The tripartite signalling system YfiBNR in P. aeruginosa modulates intracellular c-di-GMP levels in response to signals received in the periplasm and is a key regulator of the SCV phenotype. The effector protein YfiN (also known as TpbB or PA1120) is an integral inner membrane protein that functions as a diguanylate cyclase, consisting of a periplasmic PAS domain, a cytoplasmic HAMP domain and a catalytic GGDEF domain. The third component of the YfiBNR signalling system, YfiR, has a key role in the signal transduction process by bridging YfiN in the inner membrane and YfiB in the outer membrane. YfiB can release the repression of YfiN by sequestering YfiR at the outer membrane, which requires both membrane anchoring and peptidoglycan binding by YfiB for full activity.

The crystal structure of YfiR was determined to 2.40 Å resolution and reveals two molecules in an asymmetric unit, with each molecule traced in continuous electron density from Arg38 at the N-terminus to Thr189 at the C-terminus. Each YfiR monomer consists of a twisted, seven-stranded β-sheet flanked on one side by the N- and C-terminal helices (α1 and α4 respectively), and on the other by the helices α2 and α3. The mixed, seven-stranded β-sheet has a β2-β3-β1-β4-β5-β6-β7 topology. Analytical ultracentrifugation analysis confirms that YfiR forms a dimer in solution, which is consistent with a recent YfiR crystal structure. The two-fold symmetrical dimer is formed by several key interactions, including salt-bridges by Asp80 and Arg98 and main chain hydrogen bonding between Thr76 of each monomer. YfiR crystallizes as a dimer and features two pairs of conserved cysteine residues; Cys71-Cys110 are in a reduced state while Cys145-Cys152 form a disulfide bond. Two highly conserved pairs of cysteine residues were identified in the structure, Cys71-Cys110 and Cys145-Cys152, with only the latter pair confirmed to form a disulfide bond from the electron density. Mapping the conservation scores for each amino acid onto the YfiR structure reveals a large, continuous, highly conserved region on the surface of the protein formed by the C-terminal helices α3, α4 and the α3-α4 loop, with contributions from strand β7, the N-terminal helix α1 and the α1-β1 loop. The structure of P. aeruginosa YfiR was determined by single-wavelength anomalous dispersion from a Se-Met derivative protein using the AutoSol module in PHENIX with 2.25 Å data collected at the peak wavelength.

>[2x]MPSLPTLQPLDLYRRTLACLVLAVSCLGGGGLWADDARTSIEQRSNAVSQVLLGIFSYVRWPKEPAVLQLCVVGPTEYADGLLRGMVQANGRRVHAERRAVDNPDLGTLCNVIYLGVVDERERQQVFRSLAGHPVLSISERGTECSVGSMFCLNVGGPRITFEANLDSIARSGVRVHPSVLKLARRQATP> MRLHTVRAPIITRAAMRGYSEARSNYDGTSLPAWPAPGKKPTYPAALSELRLPQPRMRKTRTEWMYYHGHGGCPGKYGPSREIADFEYADGTPASISGRRFAFKHHQDHLL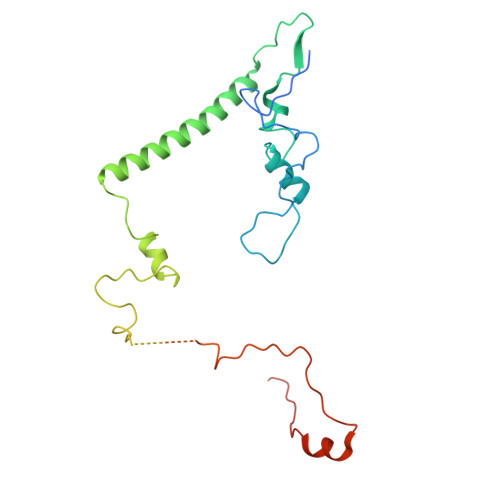VQLIRAAATVERYDASGLLPRIPGTAEQRNWDPAIPLFLDDVDEQGRPAPLRTAGDAPGTMVSHVCSRVVDERMGTPTHTPNELANRHEGETLEANTMFATNDPSAFVSDTVKLRDDKRPYWSRRRWALTDKFLVPKSPKPKNTIKDE5'-S-[(2R,4R)-1-{2-[(2-amino-7,7-dimethyl-4-oxo-3,4,7,8-tetrahydropteridine-6-carbonyl)amino]ethyl}-2-carboxypiperidin-4-yl]-5'-thioadenosine | C27 H36 N12 O7 S | 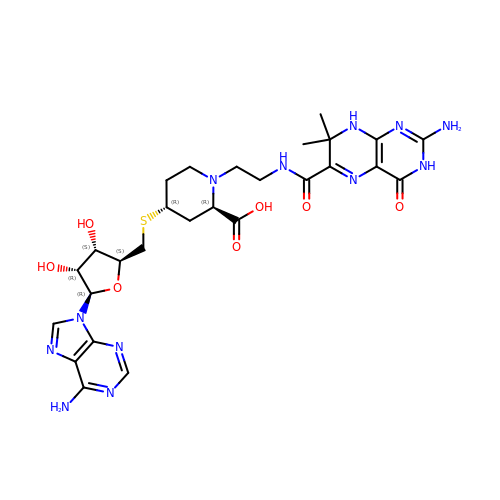DFLAELLQWVMGCU-NERDUYAPSA-N The group I mitochondrial chaperonin mHsp60 and its co-chaperonin mHsp10 assist the folding of mitochondrial-imported proteins, and correct misfolded polypeptides resulting from mitochondrial stress. Like GroEL, human mHsp60 can also assemble into stacked back-to-back double-heptameric rings capped by a dome-shaped heptameric mHsp10 (GroES in the case of E. coli) co-chaperonin lid to form ATP-driven nanocages for a substrate–protein to fold in confinement. Features shared by all three structures include mHsp60 protomers in an extended conformation along the molecular symmetry axis with clearly defined domains, namely an equatorial ATP-binding domain (residues 1–137, 411–526), an intermediate hinge domain (residues 138–191, 375–411), and an apical domain (residues 192–374). Each mHsp10 protomer adopts the canonical seven-strand β-barrel structure and exposes a flexible loop sequence of twenty residues (mobile loop) that mediates the interaction with helices H and I of the mHsp60 apical domains.

For the ADP football (stage IV), we conclude with confidence, as a result of the high resolution and quality of our cryo-EM map, that the nucleotide-binding sites in all fourteen mHsp60 subunits in both symmetric halves of the football are occupied by ADP and Mg2+, with no evidence for the presence of γ phosphate or K+. The specific amino acid interactions with ADP and Mg2+ mirror those reported in the ADP-bound crystal mHsp60E321K–mHsp10 structure, except that in our map several water molecules are also visible. To this end, we built a refined structure model from a 3D reconstruction at 3.74 Å resolution determined without imposing any symmetry (C1 symmetry). The conformational analysis described above showed the unsymmetrized cryo-EM structure displays perfect symmetry, indicating that in solution the ADP-bound football does not display subunit conformational asymmetry. In contrast, the ADP football has lost the left interaction locus, and the double mHsp60 rings are held together solely by the S464 interaction. Concomitantly, the equatorial gap has increased to 4.6 Å with the buried surface area diminished, consistent with a football poised to split into its two halves. Further, when we superimposed the ADP:BeF3 and ADP football structures, we discern a subtle but distinct concerted pivot of the ADP equatorial domains away from the interface plane, abrogating the left locus and giving rise to the single point S464 interaction. While density for the complete GGM tail is not visible in our structures, in line with the fact that this region is predicted to be unstructured, we did observe extended density radiating into the center of the ring for the ADP football. From our cryo-EM images showing abundant ADP-bound football and half-football complexes, we postulated the former might represent a pre-split intermediate.

>[14x]GQAFRKFLPLFDRVLVERSAAETVTKGGIMLPEKSQGKVLQATVVAVGSGSKGKGGEIQPVSVKVGDKVLLPEYGGTKVVLDDKDYFLFRDGDILGKYVD;>GSAKDVKFGADARALMLQGVDLLADAVAVTMGPKGRTVIIEQSWGSPKVTKDGVTVAKSIDLKDKYKNIGAKLVQDVANNTNEEAGDGTTTATVLARSIAKEGFEKISKGANPVEIRRGVMLAVDAVIAELKKQSKPVTTPEEIAQVATISANGDKEIGNIISDAMKKVGRKGVITVKDGKTLNDELEIIEGMKFDRGYISPYFINTSKGQKCEFQDAYVLLSEKKISSIQSIVPALEIANAHRKPLVIIAEDVDGEALSTLVLNRLKVGLQVVAVKAPGFGDNRKNQLKDMAIATGGAVFGEEGLTLNLEDVQPHDLGKVGEVIVTKDDAMLLKGKGDKAQIEKRIQEIIEQLDVTTSEYEKEKLNERLAKLSDGVAVLKVGGTSDVEVNEKKDRVTDALNATRAAVEEGIVLGGGCALLRCIPALDSLTPANEDQKIGIEIIKRTLKIPAMTIAKNAGVEGSLIVEKIMQSSSEVGYDAMAGDFVNMVEKGIIDPTKVVRTALLDAAGVASLLTTAEVVVTEIPKE[14x]> MSAEVIHQVEEALDTDEKEMLLFLCRDVAIDVVPPNVRDLLDILRERGKLSVGDLAELLYRVRRFDLLKRILKMDRKAVETHLLRNPHLVSDYRVLMAEIGEDLDKSDVSSLIFLMKDYMGRGKISKEKSFLDLVVELEKLNLVAPDQ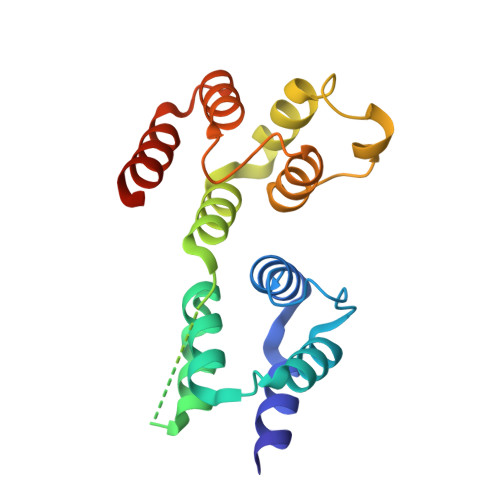LDLLEKCLKNIHRIDLKTKIQKYKQSVQGAGTS> MANVNKVVRRRQVALLIALVLGIGAGGAGTWMVSEMNLKKAPPAKAPKGEPAPDMTGVVNQSFDNKVQRSAIAEAQRLNKETQTEIKKLRTEMGLVSRDLKGSQDRIRELEDQNQLLQTQLEAGKNFDSLSAEPLPGALASQGKPAPAGNVPPPTSFWPAGGGQAPAAPVMTPIQR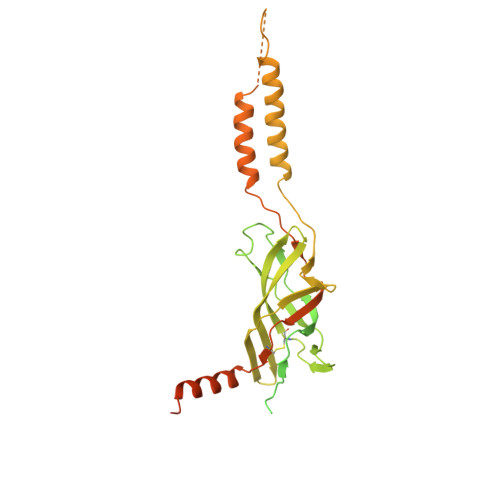PGMMDSQEFSLPDTGPKKPRFPWISSGSFVEAIVVEGADANASVTGDKNTAPMQLRLTGKVQMPNDEEFDLTGCFVTLEAWGDVSSERAIVRSRSISCKLGDDDIDQKIAGHVSFMGKNGIKGEVVMRNGQILLYAGGAGFLDGIGKGIEKASSTTVGVGATASMSAADIGQAGLGGGVSSAAKTLSDYYIKRAEQYHPVIPIGAGNEVTLVFQDGFQLETLEEARAKAAARKKQNQPSASSTPAAMPGNTPDMLKQLQDFRVGDTVDPATGQVVTQ>GHMNPIVELFIKDFTKEVMEENAAIFAGAGLSMSVGYVSWAKLLEPIAQEIGLDVNKENDLVSLAQYYCNENQGNRGRINQIILDEFSRKVDLTENHKILARLPIHTYWTTNYDRLIEKALEEENKIADVKYTVKQLATTKVKRDAVVYKMHGDVEHPSEAVLIKDDYEKYSIKMDPYIKALSGDLVSKTFLFVGFSFTDPNLDYILSRVRSAYERDQRRHYCLIKKEERRPDELEADFEYRVRKQELFISDLSRFNIKTIVLNNYNEITEILQRIENNIKTKTVFLSGSAVEYNHWETEHAEQFIHQLSKELIRKDFNIVSGFGLGVGSFVINGVLEELYMNQGTIDDDRLILRPFPQGKKGEEQWDKYRRDMITRTGVSIFLYGNKIDKGQVVKAKGVQSEFNISFEQNNYVVPVGATGYIAKDLWNKVNEEFETYYPGADARMKKLFGELNNEAL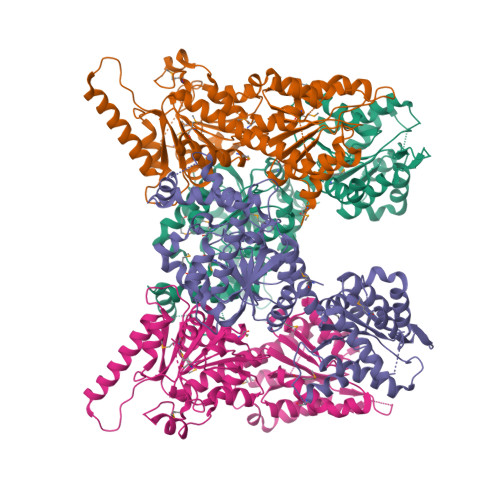SIEELINTIIEFVEILSN[4x]>[2x]MTKKVAIILANEFEDIEYSSPKEALENAGFNTVVIGDTANSEVVGKHGEKVTVDVGIAEAKPEDYDALLIPGGFSPDHLRGDTEGRYG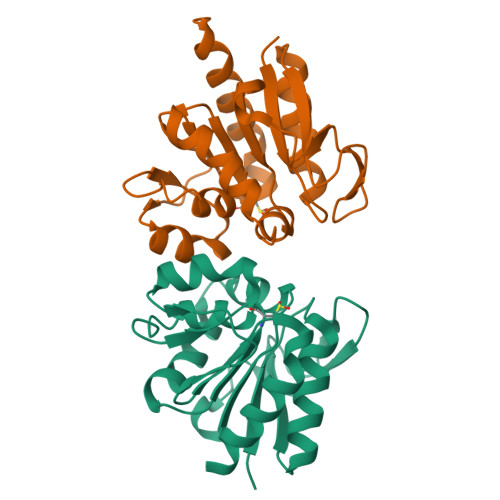TFAKYFTKNDVPTFAICHGPQILIDTDDLKGRTLTAVLNVRKDLSNAGAHVVDESVVVDNNIVTSRVPDDLDDFNREIVKQLQLEHHHHHH>GSHMTANVDGVPEKFATLGLTYDDVLLLPGASAVLPNAVDTSSRISRNVRVNIPLLSAAMDKVTESRMAISMARQGGVGVLHRNLSIEDQANQVDLVKRSESGMVANPITIHPDATLGEADALCAKFRISGVPVTDGAGKLLGIVTNRDMAFETDRSRQVREVMTPMPLVTGQVGISGVDAMELLRRHKIEKLPLVDGDGILKGLITVKDFVKAEQYPHAAKDAKGRLLVGAAVGASPEALDRAQALAEAGVDFLVVDTSHGHNSNALSWMSKIKSSVGIDVVGGNVATRDGAQALIDAGVDGIKVGVGPGSICTTRVVAGIGVPQVTAIYEASLAARAAGVPLIGDGGLQYSGDIGKALAAGADTVMLGSLLAGCEESPGELQFINGKQFKSYRGMGSLGAMQSRGQGRSYSKDRYFQAEVASDDKLVPEGIEGQVPYRGPLANVLHQLVGGLRQT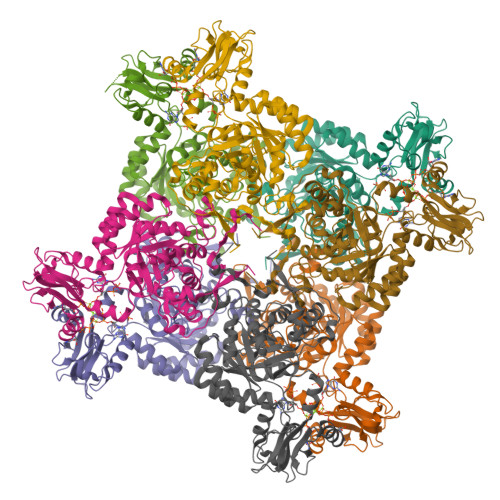MGYVGAATIEEMESKGRFVRITSAGLKESHPHDIQMTVEAPNYSRSK[16x]> HHHHHHLVPRGSPEAPYASLTEIEHLVQSVCKSYRETCQLR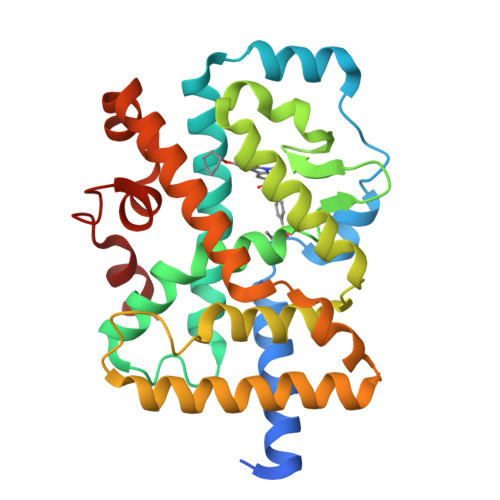LEDLLRQRSNIFSREEVTGYQRKSMWEMWERCAHHLTEAIQYVVEFAKRLSGFMELCQNDQIVLLKAGAMEVVLVRMCRAYNADNRTVFFEGKYGGMELFRALGCSELISSIFDFSHSLSALHFSEDEIALYTALVLINAHRPGLQEKRKVEQLQYNLELAFHHHLCKTHRQSILAKLPPKGKLRSLCSQHVERLQIFQHLHPIVVQAAFPPLYKELFSGGGEKHKILHRLLQDS Interestingly, human SCL (hSCL) is unlike several bacterial orthologues specific for Sec and does not accept the sulfur analogue Cys as substrate with any appreciable activity. SCL and CD enzymes are NifS-like proteins that contain a completely conserved active site Cys residue (C388, hSCL numbering) that form an enzyme-bound persulfide (Cys-S-SH) or sulfoselenide (Cys-S-Se−) as product of the reactions with Cys or Sec, respectively. Similar to the non-specific SCL/CD enzymes, hSCL was found to adopt the canonical fold type I structure of PLP enzymes, forming two active sites in the homodimer interface with each monomer contributing residues to both active sites. Structures of hSCL in two different crystal forms were determined: P1 to 1.8 Å, with four monomers per asymmetric unit and P212121 to 2.1 Å resolution, with two monomers per asymmetric unit.

Moreover, in a second crystal form (P1) of hSCL, crystallized at a higher pH of 8.1 and soaked with 10 mM Cys for 2 hours, the electron density of subunit A showed the formation of an adduct, most likely a C388-persulfide, to C388 in the closed conformation. The persulfide adduct was present in subunit A with near full occupancy and also in subunit D, but there at lower occupancy. The formation of a C388-persulfide after 2 hr incubation with 10 mM Cys is also an important clue to the chemical basis for the inherent Sec specificity of the enzyme because it indicates that hSCL is not, at least under these crystallization conditions, absolutely specific for Sec but may perform Cys desulfurization with extensive concentrations of Cys over very long time scales. However, this should have no biological relevance since the reaction rate is insignificant in activity assays. The inherent dynamic property of this segment was also confirmed by the structure in the P1 crystal form where, similar to structures of other Group-I enzymes, it was disordered to different degrees in all four monomers of the asymmetric unit. Residues A 391–394, B 386–394, C 389–393 and D 391–394 are missing from the electron density in this crystal. It appears that the dynamics of this particular protein segment is a common feature among group-I NifS-like proteins. Interestingly, in group-I enzymes, this cysteine (C388 hSCL numbering) appears universally located in a dynamic segment, shown to be able to adopt at least two ordered states in hSCL (this work). In addition, a disordered state was observed in the P1 crystal of hSCL, as previously described also for other group I enzymes.

>SMGRDAPAPAASQPSGCGKHNSPERKVYMDYNATTPLEPEVIQAMTKAMWEAWGNPSSPYSAGRKAKDIINAARESLAKMIGGKPQDIIFTSGGTESNNLVIHSVVKHFHANQTSKGHTGGHHSPVKGAKPHFITSSVEHDSIRLPLEHLVEEQVAAVTFVPVSKVSGQTEVDDILAAVRPTTRLVTIMLANNETGIVMPVPEISQRIKALNQERVAAGLPPILVHTDAAQALGKQRVDVEDLGVDFLTIVGHKFYGPRIGALYIRGLGEFTPLYPMLFGGGQERNFRPGTENTPMIAGLGKAAELVTQNCEAYEAHMRDVRDYLEERLEAEFGQKRIHLNSQFPGTQRLPNTCNFSIRGPRLQGHVVLAQCRVLMASVGAACHSDHGDQPSPVLLSYGVPFDVARNALRLSVGRSTTRAEVDLVVQDLKQAVAQLEDQA[4x]>[2x]MELIRIAMKKDLENDNSLMNKWATVAGLKNPNPLYDFLNHDGKTFNEFSSIVNIVKSQYPDREYELMKDYCLNLDVKTKAARSALEYADANMFFEIEDVLIDSMISCSNMKSKEYGKVYKIHRELSNSVITEFEAVKRLGKLNIKTPEMNSFSRLLLLYHYLSTGNFSPMAQLIKQIDLSEISE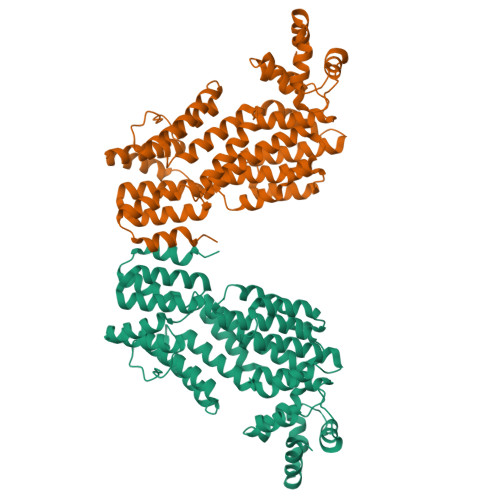NMYIRNTYQTRVHVLMSNIKLNENSLEECREYSKKALESTNILRFQVFSYLTIGNSLLFSNYELAQENFLKGLSISVQNENYNMIFQQALCFLNNVWRKENKWINFESDSIMDLQEQAHCFINFNENSKAKEVLDKLDLLVHNDNELAMHYYLKGRLEQNKACFYSSIEYFKKSNDKFLIRLPLLELQKMGENQKLLELLLLLEYA> GSHMQQQQHLHEKKRARIERARSIEGAVQVSKGTGLKNVEPRVTPKELLEWQTNWKKIMKRDSRIYFDITDDVEMNTYNKSKMDKRRDLLKRGFLTLGAQITQFFDTTVTIVITRRSV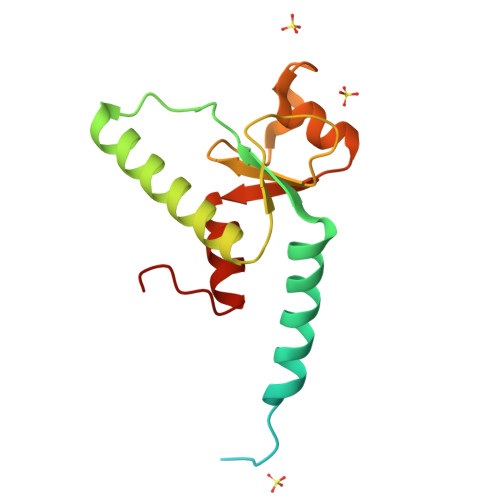ENIYLLKDTDILSRAKKNYMKVWSYEKAARFLKNLDVDLDHL>ASWSHPQFEKIEGRDTWRYAFEEAMTDVQGVYAQKFKEEIEANSDHEIQLFPYGTLGESADIMEQTQDGILQFVDQSPGFTGSLIPEAQVFFVPYLLPTDQDHLARFFKESKAINDMFKPLYADQGLELLNMFPEGEVAMTTKTPVTTCSDLDEVKFRVMTNPLLVESYKAFGATPTPLPWGEVYGGLQTNVIQGQENPTFFLYSTKIYEVTDYITYAGHNNFTTAVMANKDFYDGLSAEDQQLVQNAALAAYDHTVVYQQQAADTELAKIMEAKPE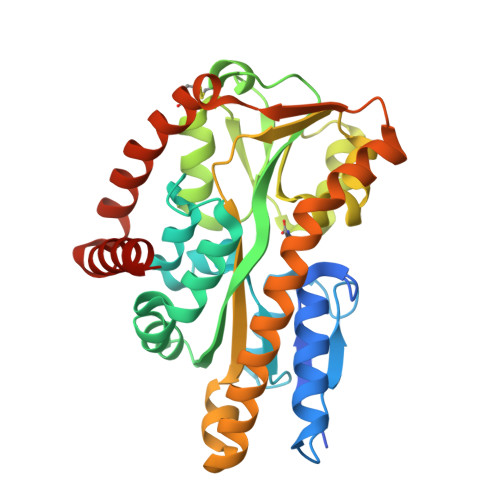MQVTVLTDEQRSCFKEAAAEVEAKFIEMTGDSGAAILKQMKADLAATAN[2x]5-acetamido-2,6-anhydro-4-carbamimidamido-3,4,5-trideoxy-3-fluoro-D-glycero-D-galacto-non-2-enonic acid | C12 H19 F N4 O7 | 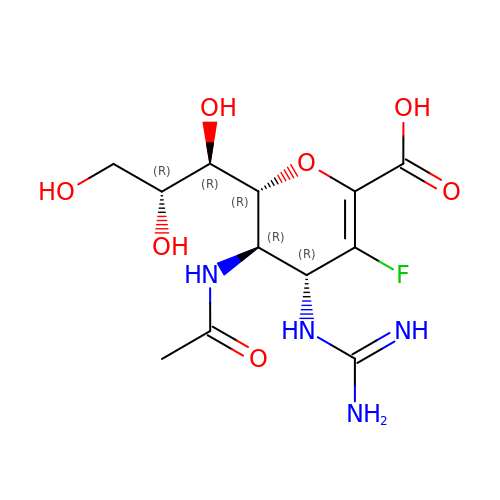UCGICVWHWQNCDB-NSNFAWTCSA-N> 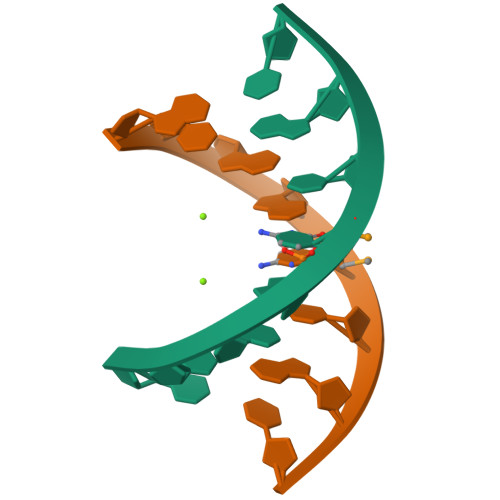GTGGCCAC> KGMTPPKTVNFKMKGVADAAF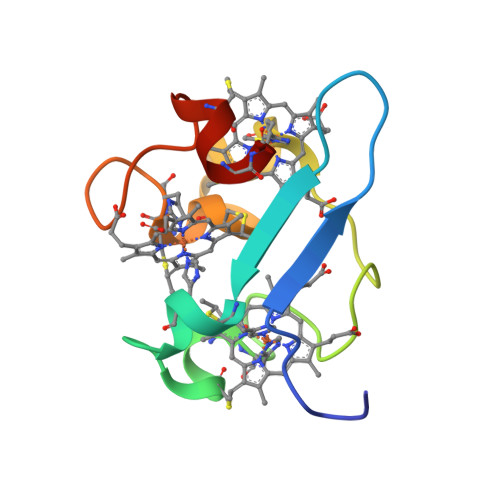SHEFHLGMYKCNECHTKLFAYKAGAKRFTMADMDKGKSCGACHNGKDAFSSASDCGKCHPG> GNP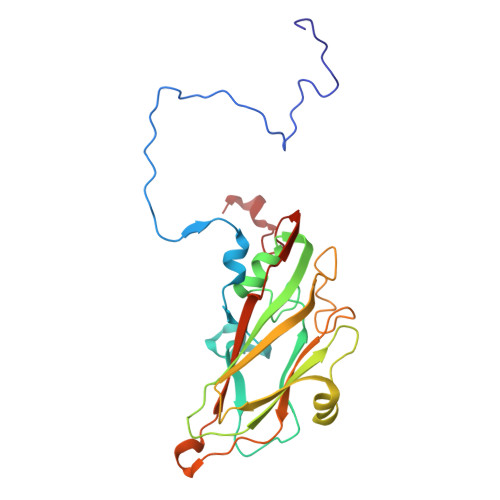TQLVPGSNMYLTSDDFRSPEAMPQFEVTPEMFIPGEVHNLMEIAETDSTVPVNNVGMAVNSMEAYRIGVNPNTGSGTQVYGWPLNPGKSSVFKRTNLGEILNYFAHWSGSIQLTFVFCGSAQATGKFLLAYSPPGAGAPTDRKGARLGTHVVWDVGLQSSCVLEVPWISNTFYRKDKSSGTGFSKAGYVTCWFQTSIVAPADAMSKCYIMCFVSADNDFSVRLLKDTPFIKEQAARRV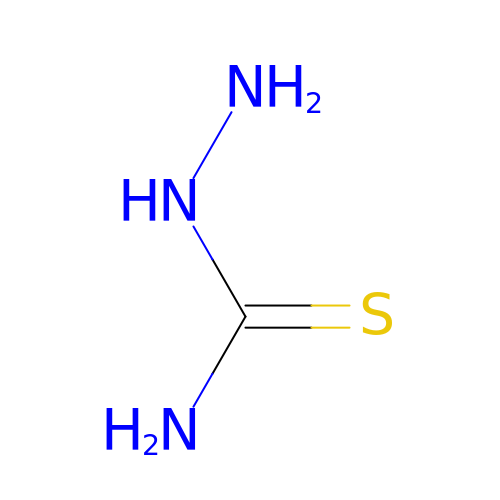HYDRAZINECARBOTHIOAMIDE | C H5 N3 S | BRWIZMBXBAOCCF-UHFFFAOYSA-N> MRSTQEERFEQRIAQETAIEPQDWMPDAYRKTLIRQIGQHAHSEIVGMLPEGNWITRAPTLRRKAILLAKVQDEAGHGLYLYSAAETLGCAREDIYQKMLDGRMKYSSIFNYPTLSWADIGVIGWLVDGAAIVNQVALCRTSYGPYARAMVKICKEESFHQRQGFEACMALAQGSEAQKQMLQDAINRFWWPALMMFGPNDDNSPNSARSLTWKIKRFTNDELRQRFVDNTVPQVEMLGMTVPDPDLHFDTESGHYRFGEIDWQEFNEVINGRGICNQERLDAKRKAWEEGTWVREAALAHAQKQHARKVA;>MGSSHHHHHHGSNQLTAYTLRLGDNCLVLSQRLGEWCGHAPELEIDLALANIGLDLLGQARNFLSYAAELAGEGDEDTLAFTRDERQFSNLLLVEQPNGNFADTIARQYFIDAWHVALFTRLMESRDPQLAAISAKAIKEARYHLRFSRGWLERLGNGTDVSGQKMQQAINKLWRFTAELFDADEIDIALSEEGIAVDPRTLRAAWEAEVFAGINEATLNVPQEQAYRTGGKKGLHTEHL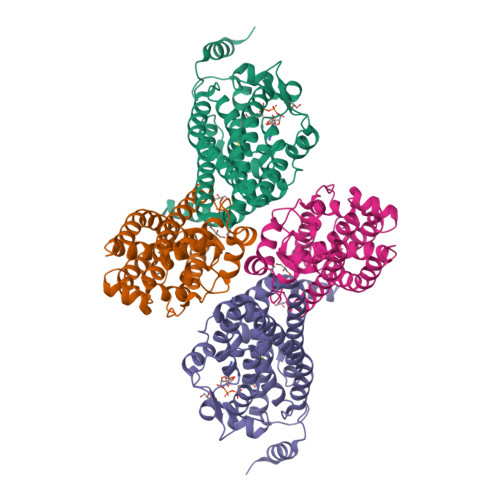GPMLAEMQYLQRVLPGQQW[2x]>[4x]GSSYDWLNALNNLELLSLHSEILTQLRSRGV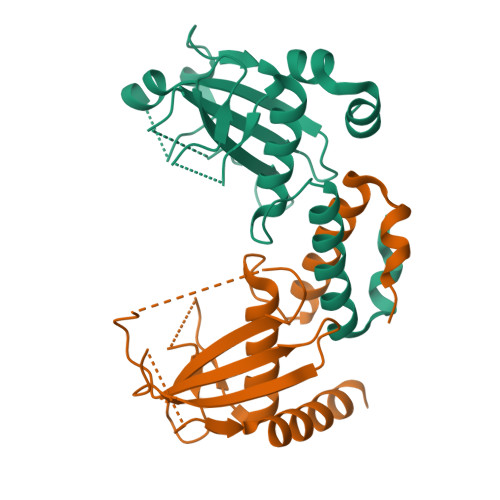IRTKNNPVGDYAEWLVSNALGMTLLSNSSAGADAIDADGLKVQIKARRVTPDNPSRQLSALRNYEAADFDYLIAVIFDETYNILDAYKIPHEVIRDYARHSDHVNAHIVNLKGAILTDPRVSSIKEDLIVRSSASVNEAAMQT>GLMDEGLPPEEVERIRAFLQERIR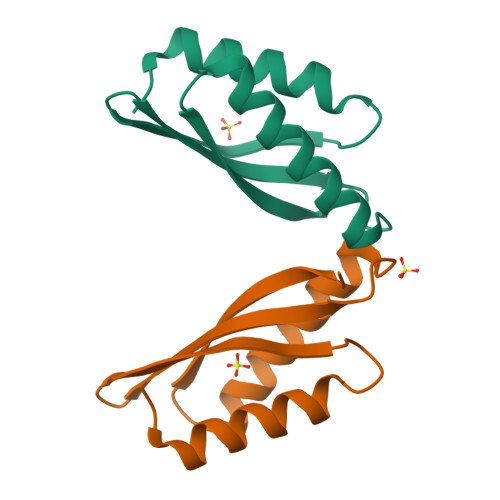GRALEVHDLKTRRAGPRSFLEFHLVVRGDTPVEEAHRLCDELERALAQAFPGLQATIHVEPEGERKRTNP[2x]> MAT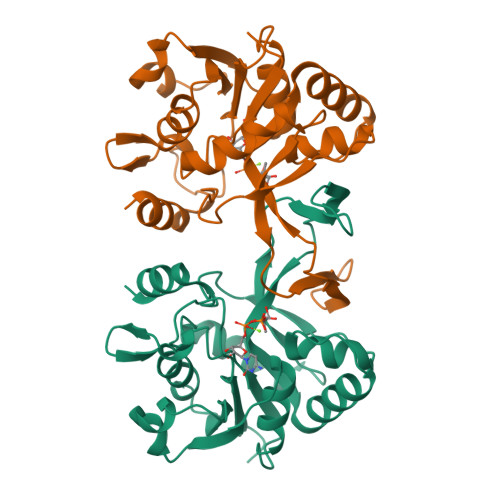THLDVCAVVPAAGFGRRMQTECPKQYLSIGNQTILEHSVHALLAHPRVKRVVIAISPGDSRFAQLPLANHPQITVVDGGDERADSVLAGLKAAGDAQWVLVHDAARPCLHQDDLARLLALSETSRTGGILAAPVRDTMKRAEPGKNAIAHTVDRNGLWHALTPQFFPRELLHDCLTRALNEGATITDEASALEYCGFHPQLVEGRADNIKVTRPEDLALAEFYLTRTIHQENT>GSHMSTITRPIIELSNTVDKIAEGNLEAEVPHQNRADEIGILAKSIERLRRSLKQLADDRTLLMAGVSHDLRTPLTRIRLATEMMSEQDGYLAESINKDIEECNAIIEQFIDYLRT[3x];> GSHMSTITRPIIELSNTVDKIAEGNLEAEVPHQNRADEIGILAKSIERLRRSLKQQADDRTLLMAGVSHDLRTPLTRIRLATEMMSEQDGYLAESINKDIEECNAI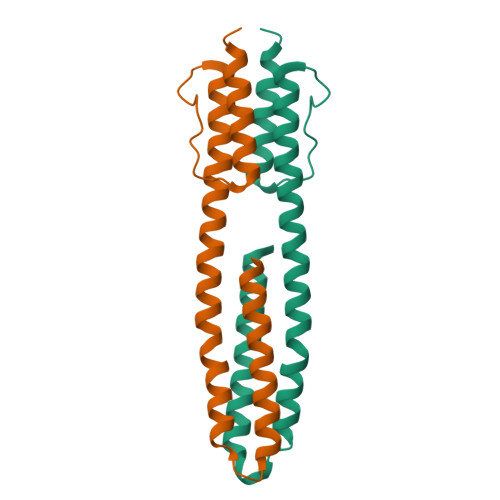IEQFIDYLRT> CRLPWNLQRI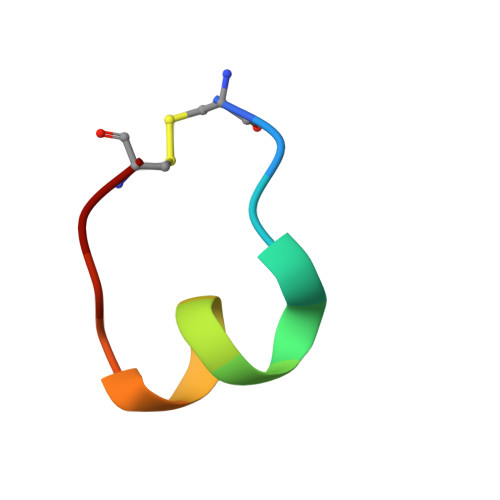GLPC(2Z)-4-oxobut-2-ene-1,2,4-tricarboxylic acid | C7 H6 O7 | 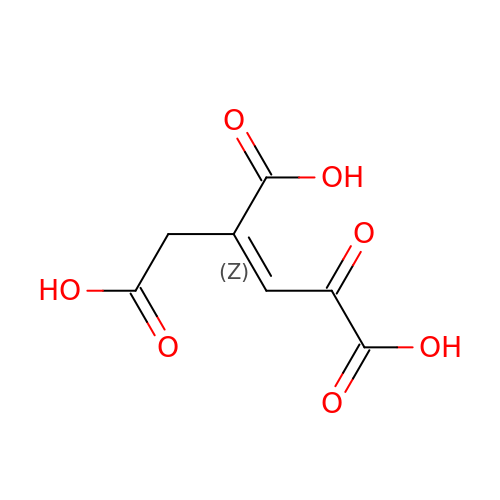POTZSFVTPSBXLW-IWQZZHSRSA-N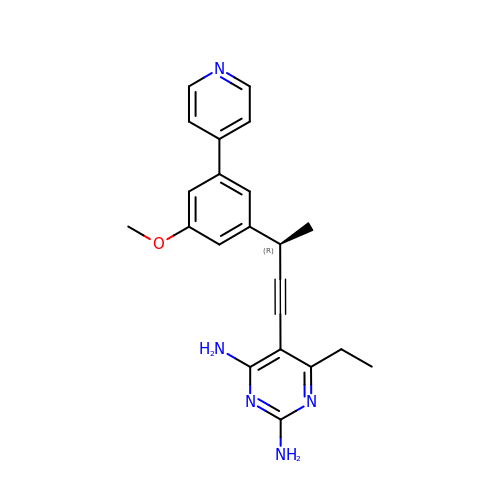6-ethyl-5-{(3R)-3-[3-methoxy-5-(pyridin-4-yl)phenyl]but-1-yn-1-yl}pyrimidine-2,4-diamine | C22 H23 N5 O | KEPLBUUTAQCZOE-AWEZNQCLSA-N> MAQTQGTRRKVCYYYDGDVGNYYYGQGHPMKPHRIRMTHNLLLNYGLYRKMEIYRPHKANAEEMTKYHSDDYIKFLRS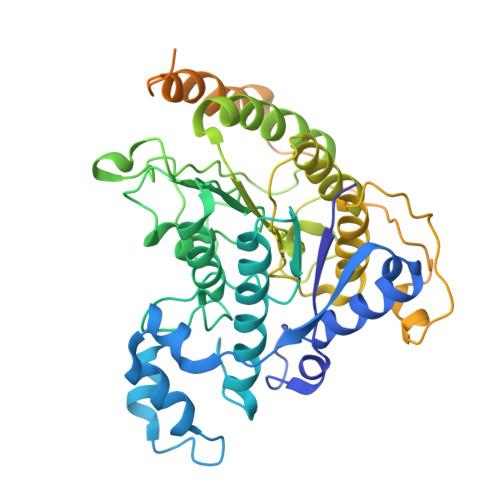IRPDNMSEYSKQMQRFNVGEDCPVFDGLFEFCQLSTGGSVASAVKLNKQQTDIAVNWAGGLHHAKKSEASGFCYVNDIVLAILELLKYHQRVLYIDIDIHHGDGVEEAFYTTDRVMTVSFHKYGEYFPGTGDLRDIGAGKGKYYAVNYPLRDGIDDESYEAIFKPVMSKVMEMFQPSAVVLQCGSDSLSGDRLGCFNLTIKGHAKCVEFVKSFNLPMLMLGGGGYTIRNVARCWTYETAVALDTEIPNELPYNDYFEYFGPDFKLHISPSNMTNQNTNEYLEKIKQRLFENLRMLPHAPGVQMQAIPEDAIPEESGDEDEDDPDKRISICSSDKRIACEEEFSDSEEEGEGGRKNSSNFKKAKRVKTEDEKEKDPEEKKEVTEEEKTKEEKPEAKGVKEEVKLA(6E,10E,14E,18E)-2,6,10,15,19,23-hexamethyltetracosa-2,6,10,14,18,22-hexaene | C30 H50 | 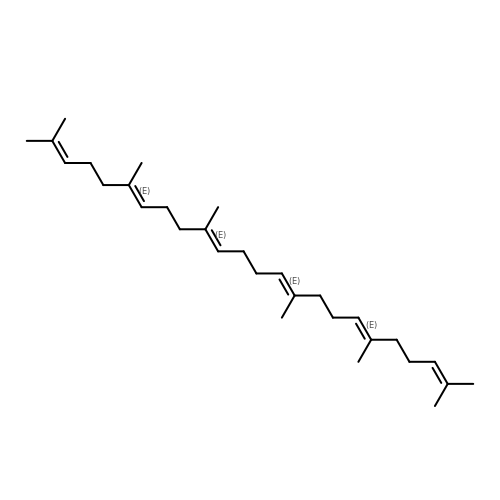YYGNTYWPHWGJRM-AAJYLUCBSA-N> MAMIEFKGKSFEIDEDGFLLKFEDWGPEWAEYVKESEGISEITEAHQQI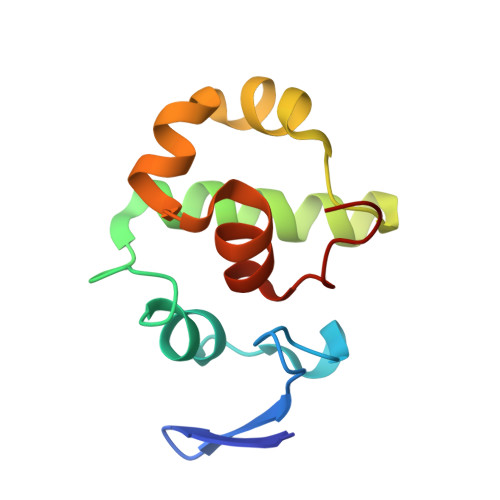LDFLQDYYKKNGIAPMVRILSKSTGYKLKQIYELFPSGPGKGACKMAGLPKPTGCV>GSMGKDEALEKDLNDVSKEINLMLSTYAKLLSERAAVDASYIDEIDELFKEANAIENALIQKREELRQRFTAIA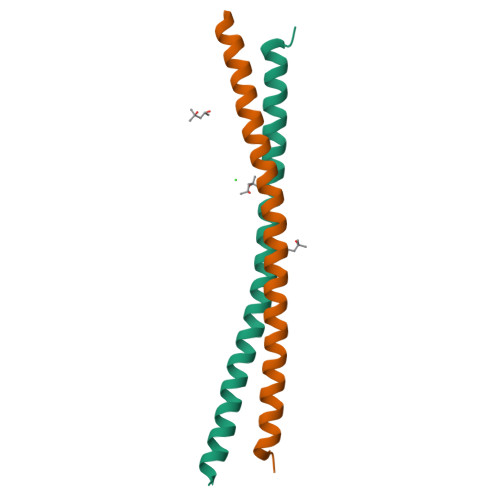NTLHR[4x]> MEGAGAGSGFRKELVSRLLHLHFKDDKTKVSGDALQLMVELLKVFVVEAAVRGVRQAQAEDALRVDV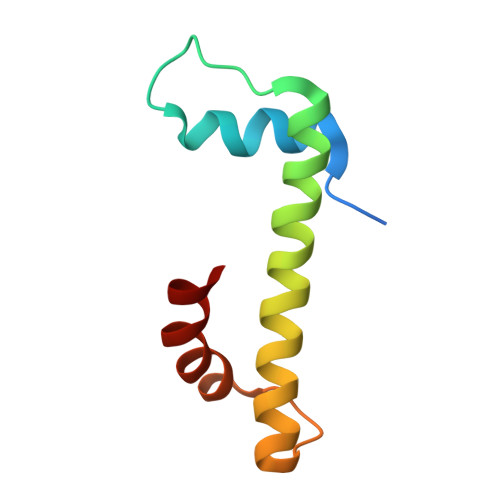DQLEKVLPQLLLDF> QPQFNEDTLQQRLQALIESAGENWTYAIFWQISHDFDSSTGDNTVILGWGDGYYKGEEDKEK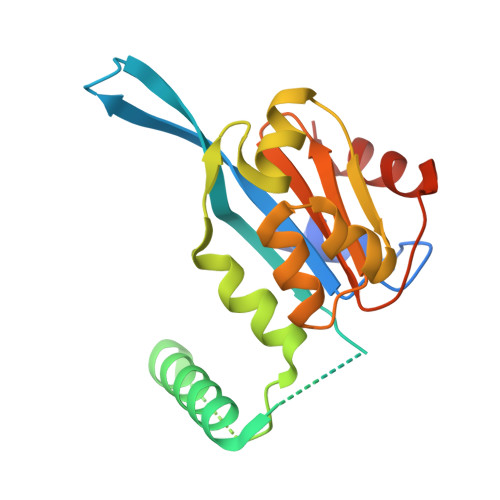KKNNTNTAEQEHRKRVIRELNSLISGGIGVSDESNDEEVTDTEWFFLVSMTQSFVNGVGLPGESFLNSRVIWLSGSGALTGSGCERAGQGQIYGLKTMVCIATQNGVVELGSSEVISQSSDLMHKVNNLFNFNNGGG> MEEKLKKTKIIFVVGGPGSGKGTQCEKIVQKYGYTHLSTGDLLRSEVSSGSARGKKLSEIMEKGQLVPLETVLDMLRDAMVAKVNTSKGFLIDGYPREVQQGEEFERRIGQPTLLLYVDAGPETMTQWLL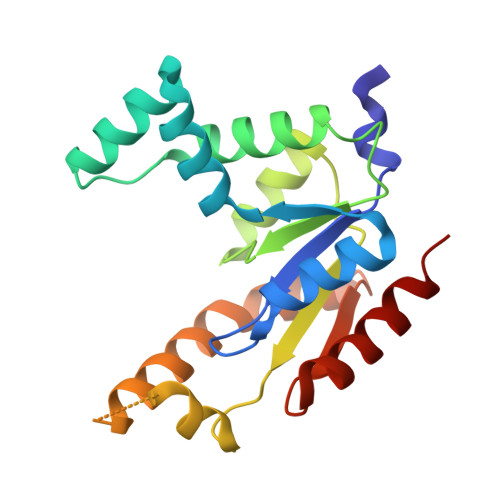KRGETSGRVDDNEETIKKRLETYYKATEPVIAFYEKRGIVRKVNAEGSVDSVFSQVCTHLDALK N-(6-cyano-3-{2-[2-(2,4-dioxo-3,4-dihydropyrimidin-1(2H)-yl)ethoxy]phenoxy}-4-methylnaphthalen-1-yl)-2-fluoro-N-methylacetamide 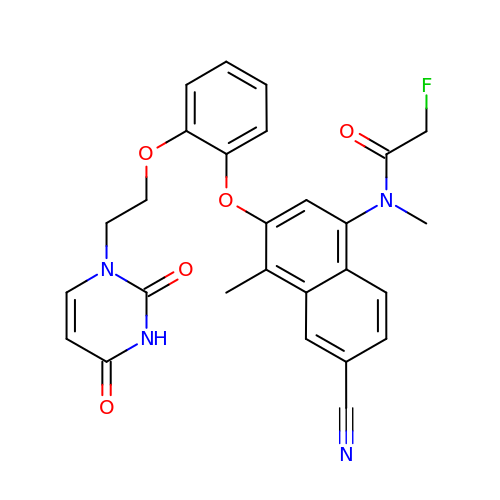| C27 H23 F N4 O5 | FGIZVIJZVLIADM-UHFFFAOYSA-N>[4x]MSEVEFSHEYWMRHALALAKRARDEREVPVGAVLVLNNRVIGEGWNRGIGLHDPTAHAEIMALRQGGLVMQNYRLYDATLYTTFEPCVMCAGAMIHSRIGRVVFGVRNAKTGAAGSLMDVLHHPGMNHRVEITEGILADECEALLCRFFRMPRRVFNAQKKAQSSTD

To confer the favorable attributes of ABEs upon a CBE, we envisioned transforming TadA into an enzyme capable of robust cytidine deamination and subsequently generated an improved class of CBEs that uses TadA instead of a naturally occurring cytidine deaminase. Here we describe the development of two families of base editors, CABE-Ts and CBE-Ts, which use variants of TadA to catalyze the deamination of cytosines with either retention (CABE-Ts) or loss (CBE-Ts) of adenine deamination. To illuminate how amino acid substitutions identified from directed evolution affect TADAC’s substrate tolerance, we determined crystal structures of TadA*8.20 from ABE8.20-m13, the template used to evolve CABE-T1, and TADAC-1 variants from CABE-T1 reported here. Through X-ray crystallography, we show how the accumulation of substitutions impacts the shape of the active site cavity and may contribute to the accommodation of cytosine as substrate and the subsequent shift in specificity toward C-to-U deamination.

Crystal structures of TadA*8.20 and TADAC-1.17 were determined in a complex with ssDNA substrate containing the adenine transition-state analog 2-deoxy-8-azanebularine (d8Az). These two structures are highly similar, and the four TADAC-1.17 substitutions (T17A, A48G, S82T and A142E) derived from evolution do not drastically alter substrate tolerance by changing the protein structure or the ssDNA binding mode. We hypothesize that the T82 side chain near the catalytic E59 residue (~4 Å) in the active site may have a role in increasing cytosine deamination by modulating proton transfer to or from E59. Additionally, the hydrogen bonding between E142 and R153 may modulate ssDNA binding by stabilizing the α6-helix, as exemplified by the interactions between F156 and dT(8) in the TADAC-1.17 structure.>VPMDTISGPWGNNGGNFWSFRPVNKINQIVISYGGGGNNPIALTFSSTKADGSKDTITVGGGGPDSITGTEMVNIGTDEYLTGISGTFGIYLDNNVLRSITFTTNLKAHGPYGQKVGTPFSSANVVG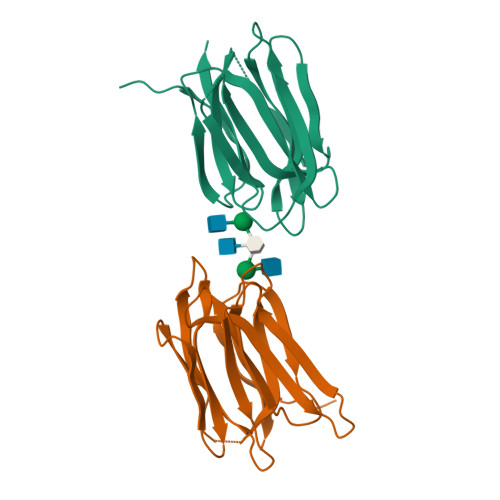NEIVGFLGRSGYYVDAIGTYNRHK[4x]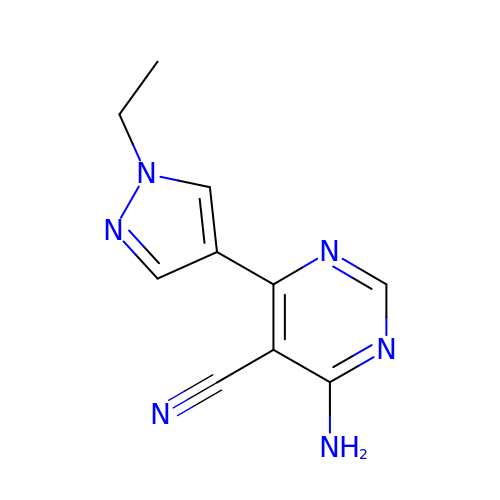4-azanyl-6-(1-ethylpyrazol-4-yl)pyrimidine-5-carbonitrile | C10 H10 N6 | UXGKYAIKFHQQGH-UHFFFAOYSA-N>[2x]MKALVRLSSN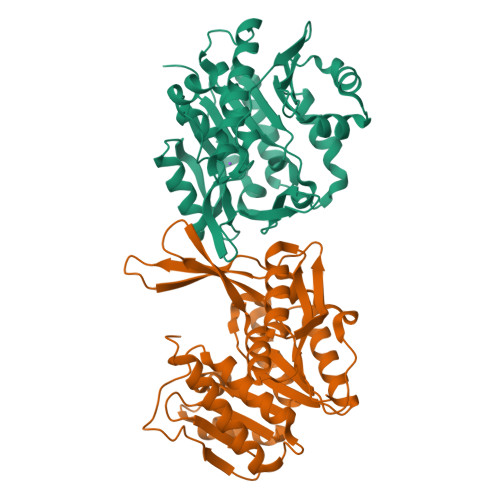HIFRSDSMSRVWLTGDAVVDLIPDGQQHYLKCPGGAPANVAVAIARLSGRSAFFGRVGNDPFGRFMQQTLTDEQVDCQHLHFDPVHRTSTVVVDLDEHGERSFTFMVKPSADQFLQLSDIPSFQKGEWLHVCSIALANQPSRSSTFAAIAQMKEVGGYVSFDPNLREEVWSEPQELQATVMRAVGLADVVKFSEEELQFLTGTQSIEEGLQAIADFQIPLVVVTLGAKGALVATPNSQQIVSGKAVKPIDTTGAGDAFVGGLLYRLSVAQDWHNQATILDAVKWANGCGALATTQKGAMTALPNQAALYAFLE> MTHQTHTIAESNNFIVLDKYIKAEPTGDSYQSESDLERELIQDLRNQGYEFISVKSQSAMLANVREQLQNLNGVVFNDSEWRRFTEQYLDNPSDGILDKTRKIHIDYICDFIFDDERLENIYLIDKKNLMRNKVQIIQQFEQAGSHANRYDVTILVNGLPLVQIELKKRGVAIREAFNQIHRYSKESFNSENSLFKYLQLFVISNGTDTRYFANTTKRDKNSFDFTMNWAKSDNTLIKDLKDFTATCFQKHTLLNVLVNYSVFDSSQTLLVMRPYQIAATERILWKIKSSFTAKNWSKPESGGYIWHTTGSGKTLTSFKAARLATELDFIDKVFFVVDRKDLDYQTMKEYQRFSPDSVNGSENTAGLKRNLDKDDNKIIVTTIQKLNNLMKAESDLPVYNQQVVFIFDECHRSQFGEAQKNLKKKFKRYYQFGFTGTPIFPENALGSETTASVFGRELHSYVITDAIRDEKVLKFKVDYNDVRPQFKSLETETDEKKLSAAENQQAFLHPMRIQEITQYILNNFRQKTHRTFPGSKGFNAMLAVSSVDAAKAYYATFKRLQEEAANKSATYKPLRIATIFSFAANEEQNAIGEISDETFDTSAMDSSAKEFLDAAIREYNSHFKTNFSTDSNGFQNYYRDLAQRVKNQDIDLLIVVGMFLTGFDAPTLNTLFVDKNLRYHGLMQAFSRTNRIYDATKTFGNIVTFRDLERSTIDAITLFGDKNTKNVVLEKSYTEYMEGFTDAATGEAKRGFMTVVSELEQRFPDPTSIESEKEKKDFVKLFGEYLRAENILQNYDEFATLKALQQIDLSDPVAVEKFKAEHYVDDEKFAELQTIRLPADRKIQDYRSAYNDIRDWQRREKEAEKKEKSTTDWDDVVFEVDLLKSQEINLDYILGLIFEHNRQNKGKGEMIEEVKRLIRSSLGNRAKEGLVVDFIQQTNLDDLPDKASIIDAFFTFAQREQQREAEALIKEENLNEDAAKRYIRTSLKREYATENGTELNETLPKLSPLNPQYKTKKQAVFQKIVSFIEKFKGVGGKI;>[2x]MKMTSIQQRAELHRQIWQIANDVRGSVDGWDFKQYVLGALFYRFISENFSSYIEAGDDSICYAKLDDSVITDDIKDDAIKTKGYFIYPSQLFCNVAAKANTNDRLNADLNSIFVAIESSAYGYPSEADIKGLFADFDTTSNRLGNTVKDKNARLAAVLKGVEGLK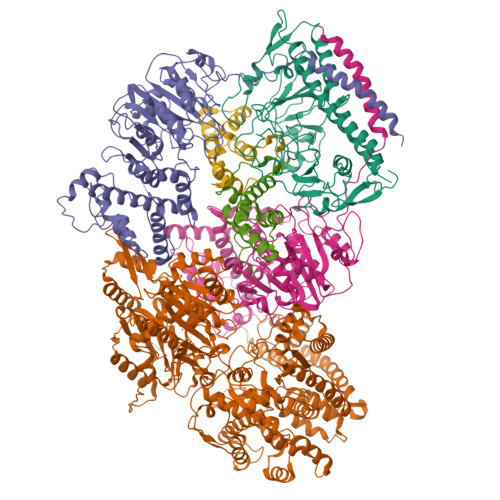LGDFNEHQIDLFGDAYEFLISNYAANAGKSGGEFFTPQHVSKLIAQLAMHGQTHVNKIYDPAAGSGSLLLQAKKQFDNHIIEEGFFGQEINHTTYNLARMNMFLHNINYDKFDIKLGNTLTEPHFRDEKPFDAIVSNPPYSVKWIGSDDPTLINDERFAPAGVLAPKSKADFAFVLHALNYLSAKGRAAIVCFPGIFYRGGAEQKIRQYLVDNNYVETVISLAPNLFFGTTIAVNILVLSKHKTDTNVQFIDASELFKKETNNNILTDAHIEQIMQVFASKEDVAHLAKSVAFETVVANDYNLSVSSYVEAKDNREIIDIAELNAELKTTVSKIDQLRKDIDAIVAEIEGCEVQK;>[2x]MAMSNMTYNNVFDHAYEMLKENIRYDDIRDTDDLHDAIHMAADNAVPHYYADIFSVMASEGIDLEFEDSGLMPDTKDVIRILQARIYEQLTIDLWEDAEDLLNEYLEEVEEYEEDEE;> MSEMSYLEKLLDGVEVEWLPLGEITKYEQPTKYLVKAKDYHDTYTIPVLTAGKTFILGYTNETHGIYQASKAPVIIFDDFTTANKWVDFDFKAKSSAMKMVTSCDDNKTLLKYVYYWLNTLPSEFAEGDHKRQWISNYSQKKIPIPCPDNPEKSLAIQSEIVRILDKFTALTAELTAELNMRKKQYNYYRDQLLSFKEGEVEWKTLGEIGKWYGGGTPSKNKIEFWENGSIPWISPKDMGRTLVDSSEDYITEEAVLHSSTKLIPANSIAIVVRSSILDKVLPSALIKVPATLNQDMKAVIPHENILVKYIYHMIGSRGSDILRAAKKTGGSVASIDSKKLFSFKIPVPNINEQQRIVEILDKFDTLTNSITEGLPREIELRQKQYEYYRDLLFSFPKPETVSN The budding yeast homologs of GBF1, named Gea1 and Gea2, localize to early and medial Golgi compartments where Arf1 activation orchestrates the formation of COPI vesicles destined for the ER and earlier Golgi compartments. Here we present cryoelectron microscopy (cryoEM) structures of full-length Gea2, the yeast paralog of the human Arf-GEF GBF1, that reveal the organization of these regulatory domains and explain how Gea2 binds to the Golgi membrane surface. Gea2 and its paralogs possess an N-terminal DCB-HUS regulatory domain and C-terminal HDS1, HDS2, and HDS3 regulatory domains. The HDS1, −2, and −3 domains form an extended helical repeat structure that is contiguous with the DCB-HUS domain, such that the HDS3 domains of each monomer lie at the distal ends of the homodimer.

Three-dimensional classification of the particles revealed three distinct conformations of Gea2 homodimers that differed only in the positioning of the GEF domain, with each monomer adopting either a “closed” or “open” position relative to the regulatory domains. Based on the relative numbers of particle images that sorted into each of these three classes (~30% “closed/closed,” ~30% “open/open,” and ~40% “closed/open”), the conformation adopted by each monomer within the dimer appears to be largely independent of that of its binding partner. Strikingly, a closed conformation of the GEF domain was not observed in the Gea2-Arf1 complex cryoEM data; instead the position of the Arf1-bound GEF domain was similar to that of the open conformation observed in the absence of Arf1. In the closed conformation the entire GEF-HDS1 linker is ordered, whereas nearly 20 residues (residue numbers 781–798) at the C-terminal end of the GEF-HDS1 linker are disordered in the open and Arf1-bound structures. For example, for a portion of the GEF-HDS1 linker in the open conformation, the cryoEM map density of some side chains is not well resolved. In contrast, the closed conformation, in which the GEF domain active site is oriented orthogonal to the membrane surface, appears much more suitable for productive encounters with the Arf1-GDP substrate via diffusion than does the open conformation. The structural data therefore suggest that the Arf1 nucleotide exchange reaction involves conformational change of its GEF from the closed state to the “open” state.

>[2x]MSDREFVTVDPVTIIIKECINLSTAMRKYSKFTSQSGVAALLGGGSEIFSNQDDYLAHTFNNLNTNKHNDPFLSGFIQLRLMLNKLKNLDNIDSLTILQPFLLIVSTSSISGYITSLALDSLQKFFTLNIINESSQNYIGAHRATVNALTHCRFEGSQQLSDDSVLLKVVFLLRSIVDSPYGDLLSNSIIYDVLQTILSLACNNRRSEVLRNAAQSTMIAVTVKIFSKLKTIEPVNVNQIYINDESYTNDVLKADTIGTNVESKEEGSQEDPIGMKVNNEEAISEDDGIEEEHIHSEKSTNGAEQLDIVQKTTRSNSRIQAYADDNYGLPVVRQYLNLLLSLIAPENELKHSYSTRIFGLELIQTALEISGDRLQLYPRLFTLISDPIFKSILFIIQNTTKLSLLQATLQLFTTLVVILGNNLQLQIELTLTRIFSILLDDGTANNSSSENKNKPSIIKELLIEQISILWTRSPSFFTSTFINFDCNLDRADVSINFLKALTKLALPESALTTTESVPPICLEGLVSLVDDMFDHMKDIDREEFGRQKNEMEILKKRDRKTEFIECTNAFNEKPKKGIPMLIEKGFIASDSDKDIAEFLFNNNNRMNKKTIGLLLCHPDKVSLLNEYIRLFDFSGLRVDEAIRILLTKFRLPGESQQIERIIEAFSSAYCENQDYDPSKISDNAEDDISTVQPDADSVFILSYSIIMLNTDLHNPQVKEHMSFEDYSGNLKGCCNHKDFPFWYLDRIYCSIRDKEIVMPEEHHGNEKWFEDAWNNLISSTTVITEIKKDTQSVMDKLTPLELLNFDRAIFKQVGPSIVSTLFNIYVVASDDHISTRMITSLDKCSYISAFFDFKDLFNDILNSIAKGTTLINSSHDDELSTLAFEYGPMPLVQIKFEDTNTEIPVSTDAVRFGRSFKGQLNTVVFFRIIRRNKDPKIFSKELWLNIVNIILTLYEDLILSPDIFPDLQKRLKLSNLPKPSPEISINKSKESKGLLSTFASYLKGDEEPTEEEIKSSKKAMECIKSSNIAASVFGNESNITADLIKTLLDSAKTEKNADNSRYFEAELLFIIELTIALFLFCKEEKELGKFILQKVFQLSHTKGLTKRTVRRMLTYKILLISLCADQTEYLSKLINDELLKKGDIFTQKFFATNQGKEFLKRLFSLTESEFYRGFLLGNENFWKFLRKVTAMKEQSESIFEYLNESIKTDSNILTNENFMWVLGLLDEISSMGAVGNHWEIEYKKLTESGHKIDKENPYKKSIELSLKSIQLTSHLLEDNNDLRKNEIFAIIQALAHQCINPCKQISEFAVVTLEQTLINKIEIPTNEMESVEELIEGGLLPLLNSSETQEDQKILISSILTIISNVYLHYLKLGKTSNETFLKILSIFNKFVEDSDIEKKLQQLILDKKSIEKGNGSSSHGSAHEQTPESNDVEIEATAPIDDNTDDDNKPKLSDVEKD> MTPPLATTIDRLRDYLDRVGFQQIYKYIVAVNHYAVTPALITRNTAASVHHFFDSRLGGRAEFALLQCLMTGRPAEHAALPDKDRALADALVTAGLLRASPDGREVSGADRQLISAFGVDLLIDRRIHFGGEVHEVYIGPASYWMLYYINASGIARTHRAVDLCTGSGIAALYLSLFTDHVLATDIGDVPLALVEINRRLNRRDAGTMEIRRENLNDTLDGRERFDLLTCNPPFVAFPPGYSGTLYSQGTGVDGLGYMRDIVGRLPEVLNPGGSAYLVADLCGDAHGPHFLGELESMVTGHGMRIEAFIDHVLPASAQVGPISDFLRHA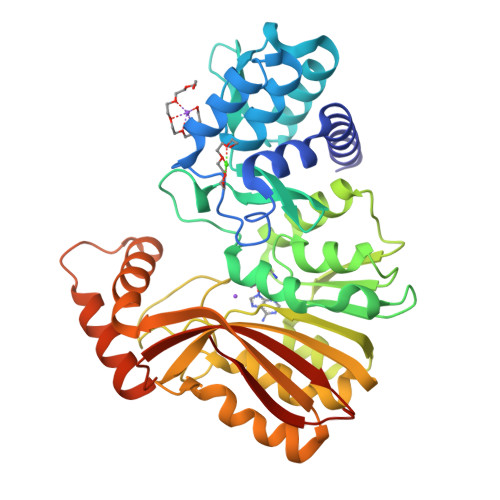AGLPADTDIAADVQAFQRETLRADYYYLTTIRLQTAAQNPGLRMLRRDPLPGAGT> APLADYKDDDDKLAGATWTTRGFVFTRHSQTTAIPSCPEGTVPLYSGFSFLFVQGNQRAHGQDLGTLGSCLQRFTTMPFLFCNVNDVCNFASRNDYSYWLSTPALMPMNMAPITGRALEPYISRCTVCEGPAIAIAVHSQTTDIPPCPHGWISLWKGFSFIMFTSAGSEGTGQALASPGSCLEEFRASPFLECHGRGTCNYYSNSYSFWLASLNPERMFRKPIPSTVKAGELEKIISRCQVCMGTGFLLVLHSQTDQEPTCPLGMPRLWTGYSLLYLEGQEKAHNQDLGLAGSCLPVFSTLPFAYCNIHQVCHYAQRNDRSYWLASAAPLPMMPLSEEAIRPYVSRCAVCEAPAQAVAVHSQDQSIPPCPQTWRSLWIGYSFLMHTGAGDQGGGQALMSPGSCLEDFRAAPFLECQGRQGTCHFFANKYSFWLTTVKADLQFSSAPAPDTLKESQAQRQKISRCQVCVAPGFLITRHSQTTDAPQCPQGTLQVYEGFSLLYVQGNKRAHGQDLGTAGSCLRRFSTMPFMFCNINNVCNFASRNDYSYWLSTPEPMPMSMQPLKGQSIQPFISRCAVCEAPAVVIAVHSQTIQIPHCPQGWDSLWIGYSFMMHTSAGAEGSGQALASPGSCLEEFRSAPFIECHGRGTCNYYANSYSFWLATVDVSDMFSKPQSETLKAGDLRTRISRCQVCMKRT

The collagen IVα345 scaffold, composed of the α3, α4, and α5 chains, is a major constituent of the GBM. The crystal structure of the hexamer revealed a ring of 12 chloride ions that, together with up to six sulfilimine bonds, stabilizes the hexamer structure. The α345 hexamer harbors a number of structural features associated with pathology, which are located within the LCL sites where pathogenic mechanisms of AS and GP converge, and potentially DN.

The single-chain α345 NC1 trimer produced recombinantly in stably transfected HEK293 cells was purified to homogeneity and crystallized in the presence of sodium chloride. The crystal structure was solved at the 1.76 Å resolution with a single polypeptide chain per asymmetric unit. It has the designed orientation of α chains in the order of α3-to-α4-to-α5. The atomic structure is homologous to the crystal structure of the α121 NC1 domain, which is also homologous to all reported crystal structures of tissue extracted from the human and bovine α121 NC1 domain. Based on sulfilimine cross-linking analysis of the GBM α345 hexamer, the expected chain pairs were α3–α5 and α4–α4 (7), although in the crystal structure, we observed α3–α3 and α4–α5 pairs. Thus, the present crystal structure of the α345 hexamer demonstrates a labile nature of a trimer–trimer orientation in the hexamer before sulfilimine cross-linking. Despite rotational mismatch of the crystallized hexamer, we discovered a set of twelve Cl- ions at the trimer–trimer interface having the same geometry as in the α121 hexamer. Geometry and residue specificity of Cl- coordination are identical between α345 and α121, with only one exception, that is, two-thirds of group 1 ions (four ions per hexamer) are not coordinated by the salt bridge to the arginine residue of the opposite trimer, rather identical arginine within the same trimer coordinates respective ions (Cl- ions #1–2). The central inner cavity going from one trimer to another through the hexamer interface accommodates multiple structured PEG molecules but would accommodate much larger molecules if present during protein folding or the hexamer assembly.> QYSPNTQQGRTSIVHLFEWRWVDIALECERYLAPKGFGGVQVSPPNENVAIYNPFRPWWERYQPVSYKLCTRSGNEDEFRNMVTRCNNVGVRIYVDAVINHMCGNAVSAGTSSTCGSYFNPGSRDFPAVPYSGWDFNDGKCKTGSGDIENYNDATQVRDCRLTGLLDLALEKDYVRSKIAEYMNHLIDIGVAGFRLDASKHMWPGDIKAILDKLHNLNSNWFPAGSKPFIYQAVIDLGGEPIKSSDYFGNGRVTEFKYGAKLGTVIRKWNGEKMSYLKNWGEGWGFVPSDRALVFVDNHDNQRGHGAGGASILTFWDARLYKMAVGFMLAHPYGFTRVMSSYRWPRQFQNGNDVNDWVGPPNNNGVIKEVTINPDTTCGNDWVCEHRWRQIRNMVIFRNVVDGQPFTNWYDN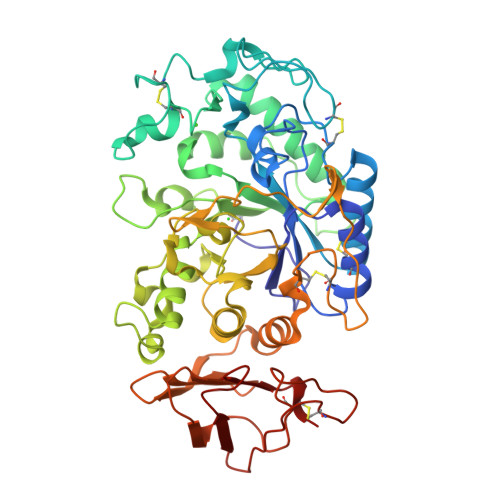GSNQVAFGRGNRGFIVFNNDDWSFSLTLQTGLPAGTYCDVISGDKINGNCTGIKIYVSDDGKAHFSISNSAEDPFIAIHAESKL>MKRIGVLTSGGDSPGMNAAIRSVVRKAIYHGVEVYGVYHGYAGLIAGNIKKLEVGDVGDIIHRGGTILYTARCPEFKTEEGQKKGIEQLKKHGIEGLVVIGGDGSYQGAKKLTEHGFPCVGVPGTIDNDIPGTDFTIGFDTALNTVIDAI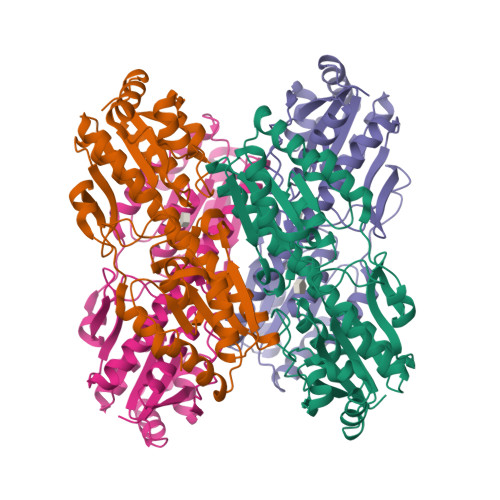DKIRDTATSHERTWVIEVMGRHAGDIALYSGLAGGAETILIPEADYDMNDVIARLKRGHERGKKHSIIIVAEGVGSGVDFGRQIQEATGFETRVTVLGHVQRGGSPTAFDRVLASRLGARAVELLLEGKGGRCVGIQNNQLVDHDIAEALANKHTIDQRMYALSKELSI[8x]> MTALPPPPSANVAVSFTAAPAEPLSRGEVKAASLKLELQNIERELKDWWMSRKILRDRNIGLFNLLQHHNFAGLSVNNA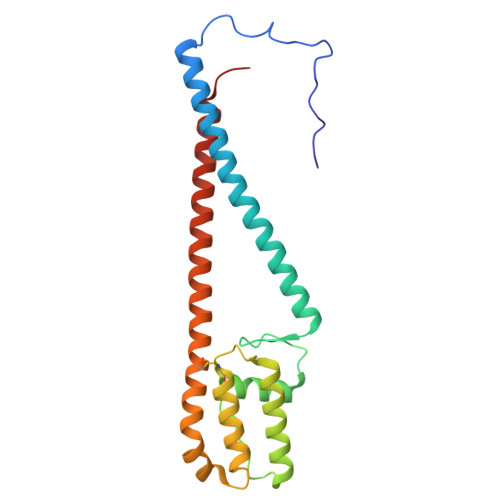KLSDSQRVMWTDLVQGKPDVEDKLSVDAREMKVDMYEKLFKQAADLENPCRMPGVAYLRCLRDTLTETQSARRSSCLNAFSSFDACRTGLLKQQSAAVENSLVRQNMADVRAKALFERRAVLLDLVEGK Aspergillus fumigatus lectin (AFL) was identified in the genome of the A. fumigatus strain Af293 by a homology search using the Aleuria aurantia lectin (AAL) from the “orange-peel” mushroom Aleuria aurantia. In conclusion, our study describes a novel fucose-specific lectin, AFL from A. fumigatus, which prefers the LeY epitope, with the ability to recognize core α1-6 Fuc. The variable composition of its binding sites enables it to bind to various fucosylated saccharides, including those expressed on human epithelia. The probable presence of AFL on the conidia and its pro-inflammatory effect makes it likely to play a role in the A. fumigatus colonization of human bodies and development of the infection.

The structure of AFL co-crystallized with methyl-α,l-selenofucoside (MeSeFuc) was determined using single-wavelength anomalous dispersion (SAD) at ESRF, Grenoble, France. The methyl-selenium used for phasing was observed on the bound fucose, as expected, but also in one residue of S-methylselenyl-l-cysteine per monomer, indicating that Cys111 received a seleniomethyl group either from SeMeFuc during soaking, or directly from the solution. The complex crystallized in the P1 spacegroup with 4 monomers per unit cell associated in 2 functional units (dimers) and the structure was refined to a resolution of 1.60 Å. The AFL monomer is composed of 6 blades, each formed of 4 antiparallel β-sheets. AFL crystallizes as a dimer that is formed by two monomers in pseudo 2-fold axial symmetry. Electron density corresponding to MeSeFuc revealed six binding sites per monomer. They are located on the opposite side of the molecule to the N- and C- termini, each of them between two adjacent blades. Binding sites are pocket-shaped, composed of different sets of amino acids, although some of them are conserved or semi-conserved. Conserved Arg and Glu/Gln residues form one side of each binding site, establishing polar contacts with the O-3, O-4 and O-5 of bound Fuc. The opposing part of each site is formed by a Trp/Tyr residue that enables hydrophobic interaction with the apolar surface of Fuc (C-3, C-4 and C-5).

>[4x]MSTPGAQQVLFRTGIAAVNSTNHLRVYFQDVYGSIRESLYEGSWANGTEKNVIGNAKLGSPVAATSKELKHIRVYTLTEGNTLQEFAYDSGTGWYNGGLGGAKFQVAPYSXIAAVFLAGTDALQLRIYAQKPDNTIQEYMWNGDGWKEGTNLGGALPGTGIGATSFRYTDYNGPSIRIWFQTDDLKLVQRAYDPHKGWYPDLVTIFDRAPPRTAIAATSFGAGNSSIYMRIYFVNSDNTIWQVCWDHGKGYHDKGTITPVIQGSEVAIISWGSFANNGPDLRLYFQNGTYISAVSEWVWNRAHGSQLGRSALPPA>GPLGSPEPDTARLDADPSASGPVMEFRELQKGAYIEPTGAFLTRARNSVSSSIPYPARAACLLVAVSQATGLPTRTLWAALCANLPDSVLDDGSLATLGLTTDHFAVLARIFSLRCRFVSEHGDVELGLHDATSRFTIRHTPGHFELVADN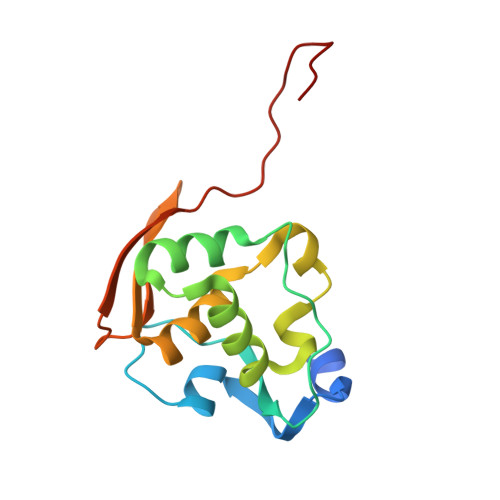FSL[2x]>MHHHHHHENLYFQSHMLLKPLQVYTADNQLIAEYGGKLSIPVEYKQIPPNFIHAFLAAEDSSFFEHSGISFKGLGRALSESVTGSDVQTGGSTITMQVAKNYYLSPERTLKRKITEIFLARKIEQNLSKEDILSLYVNKIFLGKNAYGIAAAAKIYYNKSINELSIAQMAMIAGLPKAPSKYNPVVNPERALERRNWILGRMLQLGYISQAEYQKAVAEPINLNMPNRDLNNIHPYAGEMVRSELVKHFGEQAIDSGYKVYTTINAKRQAIAEKAVQDGLEAYDRRHGWRGAEAHDKPLSEFRAYANTYPAQVTKVNSSSFEALMQDGSTVTVQWSGMSWARPYRNANSVGAAPSRASQ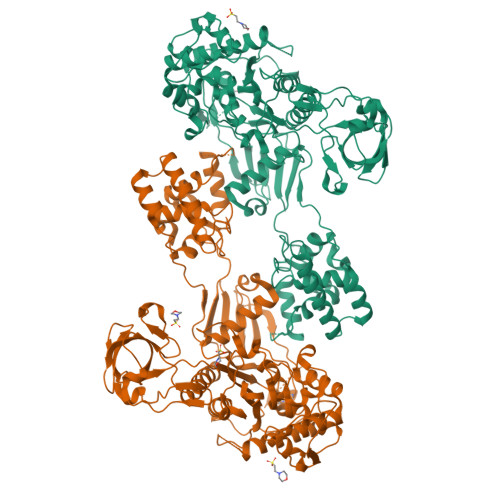IVKVKDIVRLRPNEAKTAWSLVQVPKVQGQLIAINPNDGSIEAIVGGYNFYQSKFNRALQGWRQPGSTIKPFLYALALERGMTPYSMVNDSPITIGKWTPKNSDGRYLGMIPLRRALYLSRNTVSVRLLQTVGIERTRQLFMDFGLQEDQIPRNYTIALGTPQVLPIQMATGYATFANGGYRVQPHFIQRIEDAYGKVIYEAKPEYACIPCINAPETTDDAQVTTPDDQVVEVTNKELEQKEKTTKQLNLKQTDKNNSQYRQAQRILKSSSAYDMANILRDVIEHGTGRAALKIGRSDLGGKTGTTNDAKDAWFAGFNGKLVTVTWVGFDQPTTLGRREYGGIAALPIWINFMGQALQGTPAAWVRLEKDAQ[2x]> X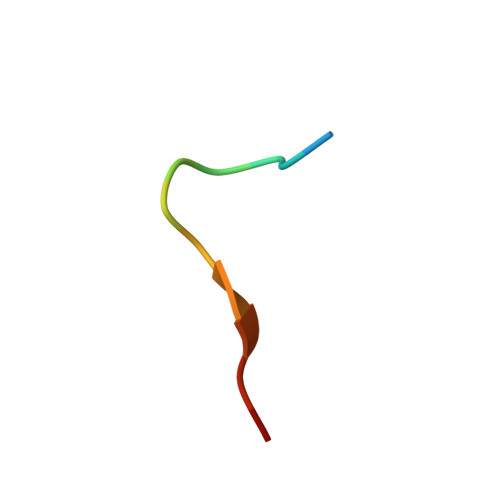WLAYPDSVPYSK> MAVSNE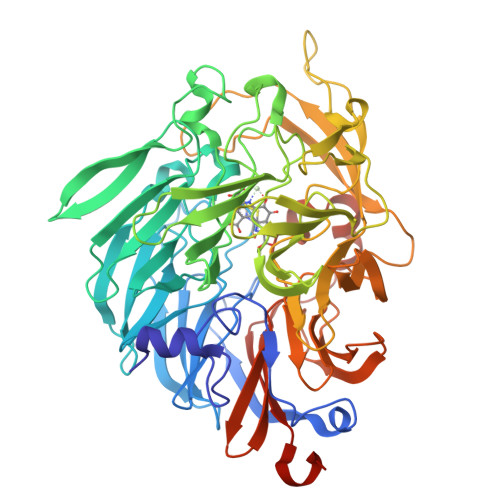EILQDPKNPQQIVTNGLGVQGQRYSPLDLLNVNNVKELRPVWAFSFGGQKQRGQQAQPLIKDGVMYLTGSYSRVFAVDARTGKKLWQYDARLPDDIRPCCDVINRGVALYGNLVFFGTLDAKLVALNKDTGKVVWSKKVADHKEGYSISAAPMIVNGKLITGVAGGEFGVVGKIQAYNPENGELLWMRPTVEGHMGYVYKDGKAIENGISGGEAGKTWPGDLWKTGGAAPWLGGYYDPETNLILFGTGNPAPWNSHLRPGDNLYSSSRLALNPDDGTIKWHFQSTPHDGWDFDGVNELISFNYKDGGKEVKAAATADRNGFFYVLDRTNGKFIRGFPFVDKITWATGLDKDGRPIYNDASRPGAPGSEAKGSSVFVAPAFLGAKNWMPMAYNKDTGLFYVPSNEWGMDIWNEGIAYKKGAAFLGAGFTIKPLNEDYIGVLRAIDPVSGKEVWRHKNYAPLWGGVLTTKGNLVFTGTPEGFLQAFNAKTGDKVWEFQTGSGVLGSPVTWEMDGEQYVSVVSGWGGAVPLWGGEVAKRVKDFNQGGMLWTFKLPKQLQQTASVKPHHHHHH N-({(1S)-5-[4-({2-[2-({2,4-BIS[HYDROXY(OXO)AMMONIO]PHENYL}AMINO)ETHOXY]ETHOXY}METHYL)-1H-1,2,3-TRIAZOL-1-YL]-1-CARBOXYPENTYL}CARBAMOYL)-L-GLUTAMIC 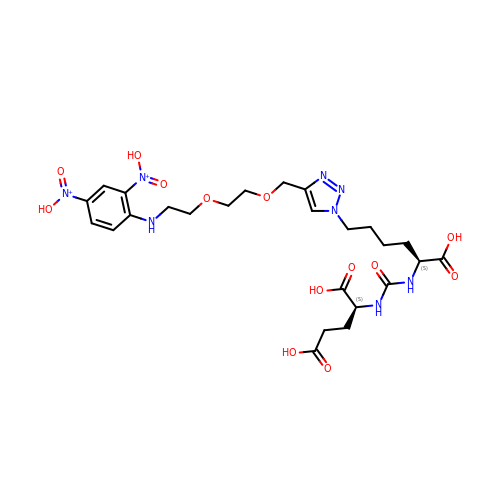ACID | C25 H36 N8 O13 | LUGMXXDMBWQRGS-PMACEKPBSA-P> GIPTELKPGTNQFLTTDDGVSAPILPGFHPTPPIHIPGEVRNLLEICRVETILEVNNLKTNETTPMQRLCFPVSVQSKTGELCAAFRADPGRDGPWQSTILGQLCRYYTQWSGSLEVTFMFAGSFMATGKMLIAYTPPGGSVPADRITAMLGTHVIWDFGLQSSVTLVVPWISNTHYRAHARAGYF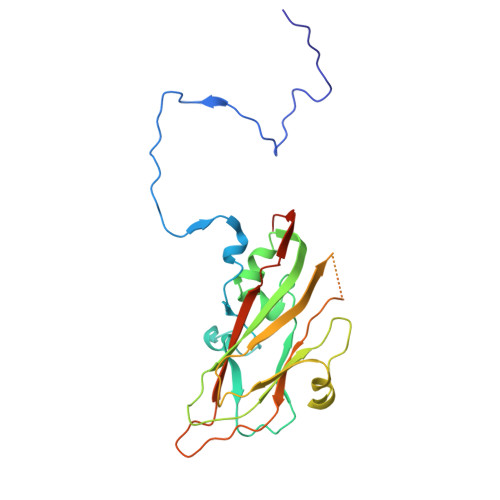DYYTTGIITIWYQTNYVVPIGAPTTAYIVALAAAQDNFTMKLCKDTEDIEQTANIQ> AQSVPYGVSQIKAPALHSEGYTGSNVKVAVIDSGIDSSHPDLKVAGGASMVPSETNPFQDNNSHGTHVAGTVAALNNSIGVLGVAPSASLYAVKVLGADGSGQYSWIINGIEWAIANNMDVINMSLGGPSGSAALKAAVDKAVASGVVVVAAAGNEGTSGSSSTVGYPGKYPSVIAVGAVDS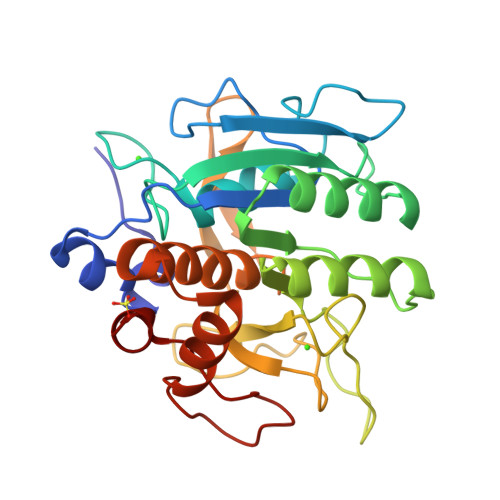SNQRASFSSVGPELDVMAPGVSIQSTLPGNKYGAYNGTSMASPHVAGAAALILSKHPNWTNTQVRSSLENTTTKLGDSFYYGKGLINVEAAAQ Escherichia coli bacteriophage T7, a member of Podoviridae, has been used as a model for understanding the DNA packaging mechanism common to tailed phages and related dsDNA viruses. The phages package genomic dsDNA into a round procapsid using the portal in complex with an ATP-dependent terminase complex as the motor. At the beginning of phage infection, the tail is responsible for receptor recognition, and the portal and tail act as a tunnel for DNA delivery into the host cytoplasm. Here, we determined structures of the DNA packaging intermediate and mature capsids of T7 using cryo-electron microscopy (cryo-EM) and symmetry-mismatch reconstruction.

Subsequently, a 7 Å resolution asymmetric reconstruction of the mature phage with a portal-tail complex at one of the 12 icosahedral vertices was obtained using the symmetry-mismatch reconstruction method. The portal-tail complex structure is similar to the previously reported recombinant T7 portal-tail complex structure. The portal-tail complex was reconstructed at the same resolution of 3.8 Å, although the core structure was still smeared. Another two independent local reconstructions focused on the portal and tail, respectively, yield the structures of the portal and tail at the same resolution of 3.8 Å, suggesting that the portal interacts firmly with the tail. Twelve copies of adaptor protein gp11 assemble around the bottom of the portal forming a ring-like structure and serving as the base for the assembly of a hexameric tube consisting of six copies of nozzle protein gp12. Six trimers of the tail fiber gp17 N-termini anchoring to the adaptor-portal interface were clearly resolved. The dsDNA is embraced by the 12 tunnel loops in the portal, which have a weaker density probably due to its asymmetric interaction with the dsDNA groove. This dsDNA density terminates abruptly at the interface between the dodecameric ring of gp11 and hexameric nozzle of gp12. The clip tilts toward the portal axis, which probably triggers the disassociation of the terminase complex, followed by the assembly of the tail proteins. It is noteworthy that If the portal does not move downward and expose its clip domain out of the capsid shell, the tail is not able to assemble on the portal due to steric restriction.

>MRSYDMNVETAAELSAVNDILASIGEPPVSTLEGDANADAANARRILNKINRQIQSRGWTFNIEEGITLLPDVYSNLIVYSDDYLSLMSTSGQSIYVNRGGYVYDRTSQSDRFDSGITVNIIRLRDYDEMPECFRYWIVTKASRQFNNRFFGAPEVEGVLQEEEDEARRLCMEYEMDYGGYNMLDGDAFTSGLLTR[12x]> GYDEIEELKSKNEVLTNLLNKLIAFDKKRIFLYPVNVQLVPDYLNVIKEPMDFTTMKQKLQNFKYKSFQEFEKDVLLIINNCYTYNDPSTIYYKFAEDIE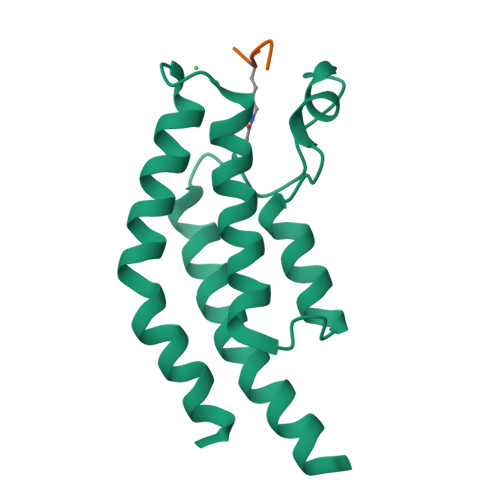TYYKKLNIKIQTKYMNIHL;> GRGKGGK> MSATKSIVGEALEYVNIGLSHFLALPLAQ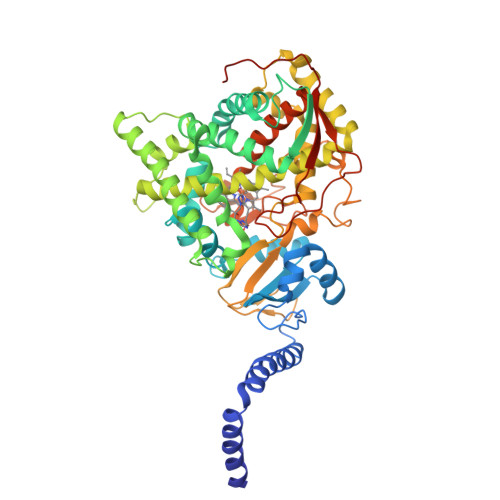RISLIIIIPFIYNIVWQLLYSLRKDRPPLVFYWIPWVGSAVVYGMKPYEFFEECQKKYGDIFSFVLLGRVMTVYLGPKGHEFVFNAKLADVSAEAAYAHLTTPVFGKGVIYDCPNSRLMEQKKFVKGALTKEAFKSYVPLIAEEVYKYFRDSKNFRLNERTTGTIDVMVTQPEMTIFTASRSLLGKEMRAKLDTDFAYLYSDLDKGFTPINFVFPNLPLEHYRKRDHAQKAISGTYMSLIKERRKNNDIQDRDLIDSLMKNSTYKDGVKMTDQEIANLLIGVLMGGQHTSAATSAWILLHLAERPDVQQELYEEQMRVLDGGKKELTYDLLQEMPLLNQTIKETLRMHHPLHSLFRKVMKDMHVPNTSYVIPAGYHVLVSPGYTHLRDEYFPNAHQFNIHRWNNDSASSYSVGEEVDYGFGAISKGVSSPYLPFSGGRHRCIGEHFAYCQLGVLMSIFIRTLKWHYPEGKTVPPPDFTSMVTLPTGPAKIIWEKRNPEQKIGGRHHHHHH>[6x]PPGTVDKKMVEKCWKLMDKVVRLCQNPKLALKNSPPYILDLLPDTYQHLRTILSRYEGKMETLGENEYFRVFMENLMKKTKQTISLFKEGKERMYEEN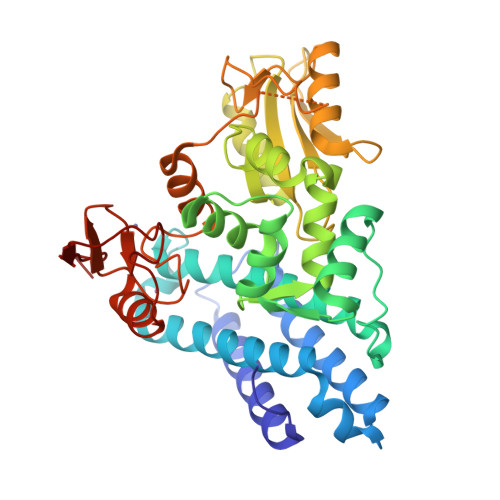SQPRRNLTKLSLIFSHMLAELKGIFPSGLFQGDTFRITKADAAEFWRKAFGEKTIVPWKSFRQALHEVHPISSGLEAMALKSTIDLTCNDYISVFEFDIFTRLFQPWSSLLRNWNSLAVTHPGYMAFLTYDEVKARLQKFIHKPGSYIFRLSCTRLGQWAIGYVTADGNILQTIPHNKPLFQALIDGFREGFYLFPDGRNQNPDLTGLCEPTPQDHIKVTQEQYELYCEMGSTFQLCKICAENDKDVKIEPCGHLMCTSCLTSWQESEGQGCPFCRCEIKGTEPIVVDPFD> GPTKAPTKDGTSYKDLFLELYGKIKDPKNGYFSPDEGIPYHSIETLIVEAPDYGHVTTSEAFSYYVWLEAMYGNLTGNWSGVETAWKVMEDWIIPDSTEQPGMSS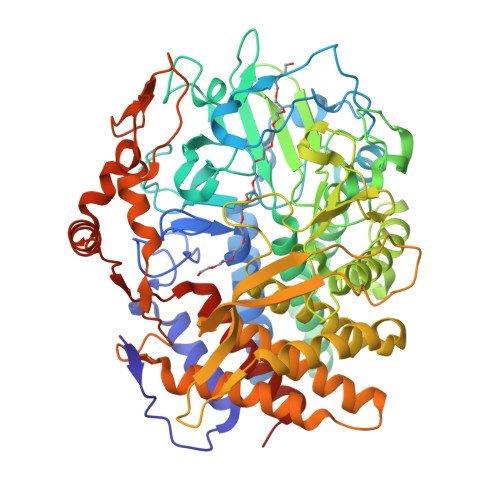YNPNSPATYADEYEDPSYYPSELKFDTVRVGSDPVHNDLVSAYGPNMYLMHWLMDVDNWYGFGTGTQATFINTFQRGEQESTWETIPHPSIEEFKYGGPNGFLDLFTKDRSYARQWRYTNAPDAEGRAIQAVYWANKWAKEQGKGSAVASVVSKAAKMGDFLRNDMFDKYFMKIGAQDKTPATGYDSAHYLMAWYTSWGGGIGASWAWKIGCSHAHFGYQNPFQGWVSATQSDFAPKSSNGKRDWTTSYKRQLEFYQWLQSAEGAIAGGATNSWNGRYEKYPAGTSTFYGMAYVPHPVYADPGSNQWFGFQAWSMQRVMEYYLETGDSSVKNLIKKWVDWVMSEIKLYDDGTFAIPSDLEWSGQPDTWTGTYTGNPNLHVRVTSYGTDLGVAGSLANALATYAAATERWEGKLDTKARDMAAELVNRAWYNFYCSEGKGVVTEEARADYKRFFEQEVYVPAGWSGTMPNGDKIQPGIKFIDIRTKYRQDPYYDIVYQAYLRGEAPVLNYHRFWHEVDLAVAMGVLATYFPDGGGGGRPHHHHHHHHHHHH(1~{R},3~{S})-~{N}-(6,7-dimethoxy-2-oxidanylidene-chromen-3-yl)-3-[(phenylmethyl)amino]cyclohexane-1-carboxamide 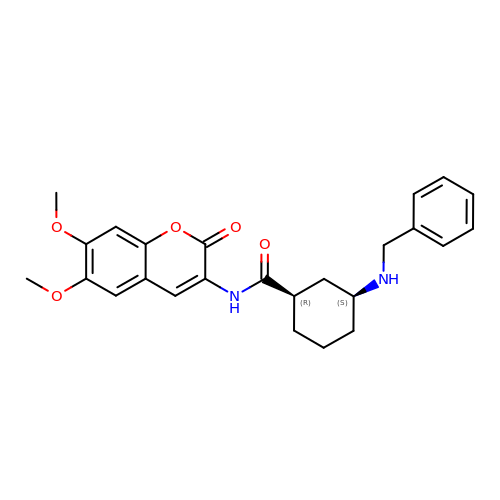| C25 H28 N2 O5 | UGTGSTDFYWUXNH-MJGOQNOKSA-N> MEINPYLMFLNNDVTSLISTTYPYTGPPPMSHGSSTKYTLETIKRTYDYSRTSVEKTSKVFNIPRRKFCNCLEDKDELVKPTGNVDISSLLGLAEMMEKRMGEGFFKHCVMEAETEILKMHFSRLTEGRQTYDWTSERNMPAATALQLTVDAIKETEGPFKGTTMLEYCNKMIEMLDWKEIKFKKVKTVVRREKDKRSGKEIKTKVPVMGID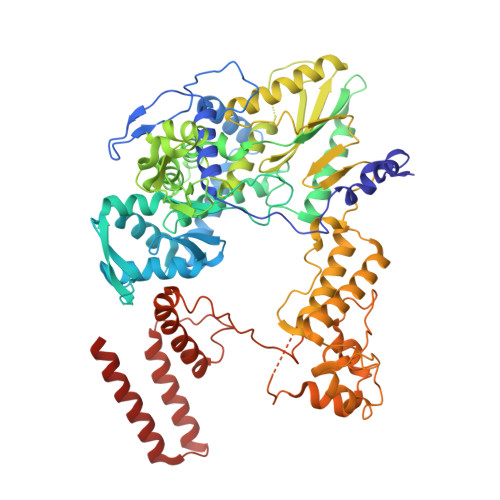SIKHDEFLIRALTINTMAKDGERGKLQRRAIATPGMIVRPFSKIVETVAQKICEKLKESGLPVGGNEKKAKLKTTVTSLNARMNSDQFAVNITGDNSKWNECQQPEAYLALLAYITKDSSDLMKDLCSVAPVLFCNKFVKLGQGIRLSNKRKTKEVIIKAEKMGKYKNLMREEYKNLFEPLEKYIQKDVCFLPGGMLMGMFNMLSTVLGVSTLCYMDEELKAKGCFWTGLQSSDDFVLFAVASNWSNIHWTIRRFNAVCKLIGINMSLEKSYGSLPELFEFTSMFFDGEFVSNLAMELPAFTTAGVNEGVDFTAAMSIIKTNMINNSLSPSTALMALRICLQEFRATYRVHPWDSRVKGGRMKIINEFIKTIENKDGLLIADGGKLMNNISTLHIPEEVLKFEKMDEQYRNRVFNPKNPFTNFDKTIDIFRAHGPIRVEENEAVVSTHSFRTRANRTLLNTDMRAMMAEEKRYQMVCDMFKSVFESADINPPIGAMSIGEAIEEKLLERAKMKRDIGAIEDSEYEEIKDIIRDAKKARLESR>GTIYPRNPAMYSEEARLKSFQN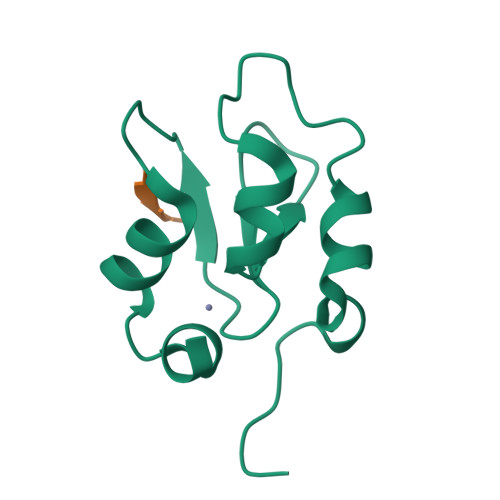WPDYAHLTPRELASAGLYYTGIGDQVQCFACGGKLKNWEPGDRAWSEHRRHFPNCFFVLGRNLN[2x];> SVPI>[2x]SNAMAEIKITPEELERIAGNFKNAAGEAQSQINR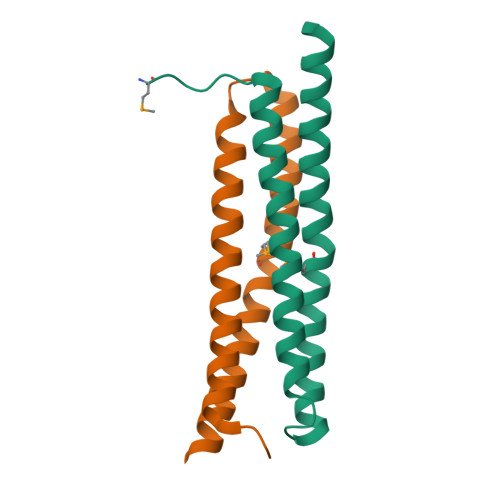LEGDINSLEGQWAGATQAKFRGEFIQSKQAMQQYIPILEGISTDLKRIADKFRNTDNAY>SHGSMTNKELQAIRKLLMLDVSEAAEHIGRVSARSWQYWESGRSAVPDDVEQEMLDLASVRIEMMSAIDKRLADGERPKLRFYNKLDEYLADNPDHNVIGWRLSQSVAALYY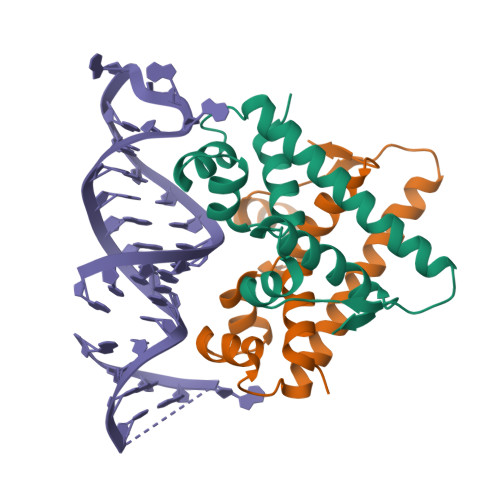TEGHADLI[2x]>[2x]MHHHHHHGSTSLYKKAGSETLYIQGMAEFPASLLILNGKSTDNLPLREAIMLLREEGMTIHVRVTWEKGDAARYVEEARKFGVATVIAGGGDGTINEVSTALIQCEGDDIPAL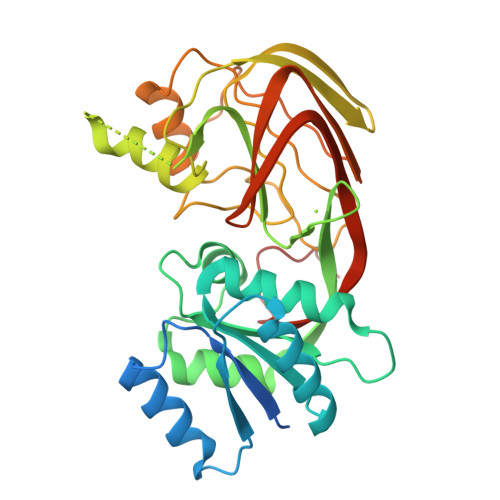GILPLGTANDFATSVGIPEALDKALKLAIAGDAIAIDMAQVNKQTCFINMATGGFGTRITTETPEKLKAALGSVSYIIHGLMRMDTLQPDRCEIRGENFHWQGDALVIGIGNGRQAGGGQQLCPNALINDGLLQLRIFTGDEILPALVSTLKSDEDNPNIIEGASSWFDIQAPHDITFNLDGEPLSGQNFHIEILPAALRCRLPPDCPLLRSTHHHHHH>[3x]MTEPSLSPAVQTFWKWLQEEGVITAKTPVKASVVTEGLGLVALKDISRNDVILQVPKRLWI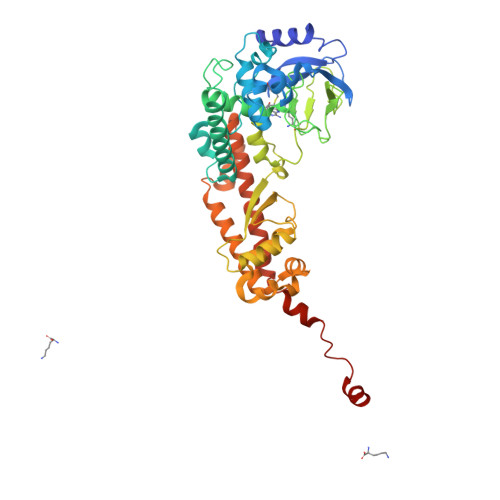NPDAVAASEIGRVCSELKPWLSVILFLIRERSREDSVWKHYFGILPQETDSTIYWSEEELQELQGSQLLKTTVSVKEYVKNECLKLEQEIILPNKRLFPDPVTLDDFFWAFGILRSRAFSRLRNENLVVVPMADLINHSAGVTTEDHAYEVKGAAGLFSWDYLFSLKSPLSVKAGEQVYIQYDLNKSNAELALDYGFIEPNENRHAYTLTLEISESDPFFDDKLDVAESNGFAQTAYFDIFYNRTLPPGLLPYLRLVALGGTDAFLLESLFRDTIWGHLELSVSRDNEELLCKAVREACKSALAGYHTTIEQDRELKEGNLDSRLAIAVGIREGEKMVLQQIDGIFEQKELELDQLEYYQERRLKDLGLCGENGDILENLYFQ>[2x]MIQFSINRTLFIHALNTTKRAISTKNAIPILSSIKIEVTSTGVTLTGSNGQISIENTIPVSNENAGLLITSPGAILLEASFFINIISSLPDISINVKEIEQHQVVLTSGKSEITLKGKDVDQYPRLQEVSTENPLILKTKLLKSIIAETAFAASLQESRPILTGVHIVLSNHKDFKAVATDSHRMSQRLITLDNTSADFMVVLPSKSLREFSAVFTDDIETVEVFFSPSQILFRSEHISFYTRLLEGNYPDTDRLLMTEFETEVVFNTQSLRHAMERAFLISNATQNGTVKLEITQNHISAHVNSPEVGKVNEDLDIVSQSGSDLTISFNPTYLIESLKAIKSETVKIHFLSPVRPFTLTPGDEEESFIQLITPVRTN

Sliding DNA clamps are processivity factors that are required for efficient DNA replication. The β subunit of the holoenzyme is required for efficient processivity in bacteria. This protein factor wraps around double-stranded DNA at primer-template junctions, where it serves as a sliding clamp to tether the polymerase enzyme to its DNA substrate. Here we present the crystal structure of the β subunit of DNA polymerase III from Streptococcus pyogenes, a Gram-positive bacterium.

The crystal structure of the β subunit from Streptococcus pyogenes was determined by multiple anomalous diffraction (MAD) at 2.6 Å resolution using datasets for three separate wavelengths close to the selenium absorption edge. A model built into the phased electron density maps was refined subsequently to 2.1 Å resolution against native data. These crystals (space group P21) contain one β dimer in the asymmetric unit. Consistent with the structure of the E. coli β clamp, the S. pyogenes clamp dimer is formed in a head-to-tail fashion. Interestingly, the S. pyogenes β clamp dimer has a distorted oval shape, unlike the more circular shape of the E. coli β clamp. The longer of the outer oval diameters is ~90 Å while the shortest diameter across the clamp is ~65 Å. The overall organization of the S. pyogenes β subunit is very similar to that of the E. coli β subunit, with three distinct domains in each protomer. The interior of the central hole in the S. pyogenes clamp is lined with basic residues, many of which (e.g., Arg 8, Lys 25, Lys 143, Lys 206, Arg 272, and Lys 342) are conserved between the S. pyogenes and the E. coli proteins. In the closed form of the S. pyogenes β clamp, helix α1" displays an even larger displacement from ideal geometry in comparison to the E. coli β clamp. This distortion of the interface in the S. pyogenes clamp is correlated with the presence of the sidechain of Phe 81, which pushes against helix α1".quinolin-8-yl piperidine-1-carboxylate | C15 H16 N2 O2 | 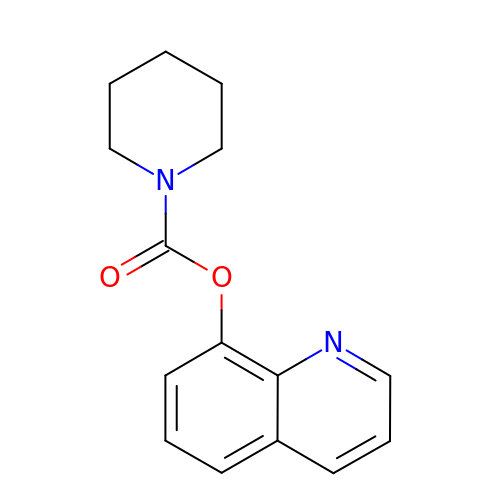NMAHWWYZVAQAMR-UHFFFAOYSA-N>SNAMTIRFADKADCAAITEIYNHAVLHTAAIWNDRTVDTDNRLAWYEARQLLGYPVLVSEENGVVTGYASFGDWRSFDGFRYTVEHSVYVHPAHQGKGLGRKLLSRLIDEARRCGKHVMVAGIESQNAASIRLHHSLGFTVTAQMPQVGVKFGRWLDLTFMQLQL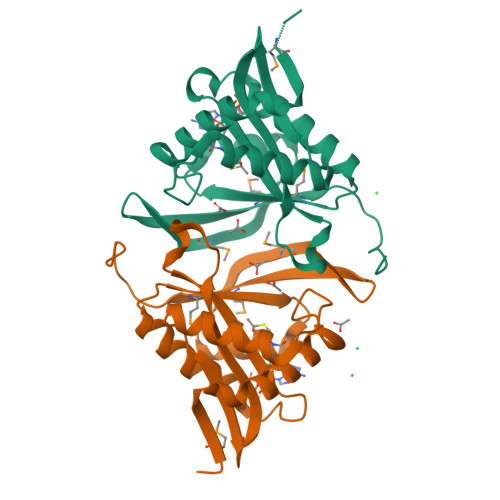DEHAAPDAC[2x]>[4x]MTIGIDKINFYVPKYYV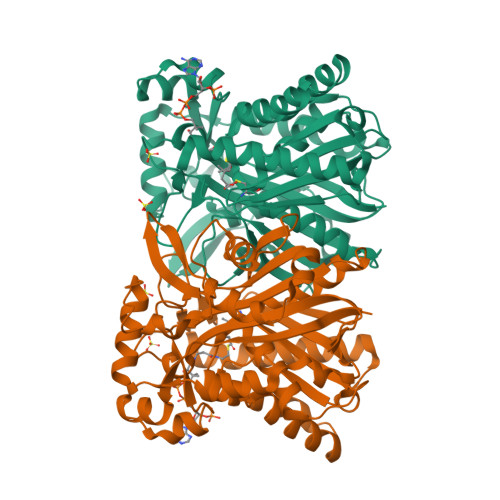DMAKLAEARQVDPNKFLIGIGQTEMAVSPVNQDIVSMGANAAKDIITDEDKKKIGMVIVATESAVDAAKAAAVQIHNLLGIQPFARCFEMKEACYAATPAIQLAKDYLATRPNEKVLVIATDTARYGLNSGGEPTQGAGAVAMVIAHNPSILALNEDAVAYTEDVYDFWRPTGHKYPLVDGALSKDAYIRSFQQSWNEYAKRQGKSLADFASLCFHVPFTKMGKKALESIIDNADETTQERLRSGYEDAVDYNRYVGNIYTGSLYLSLISLLENRDLQAGETIGLFSYGSGSVGEFYSATLVEGYKDHLDQAAHKALLNNRTEVSVDAYETFFKRFDDVEFDEEQDAVHEDRHIFYLSNIENNVREYHRPE Bestrophin-1 (Best1) and bestrophin-2 (Best2) are two members of the bestrophin family of calcium (Ca2+)-activated chloride (Cl−) channels with critical involvement in ocular physiology and direct pathological relevance. The bestrophins are a family of Ca2+-activated anion channels consisting of four members (Best1–4) in mammals. The overall architecture of hBest1 and hBest2 resembles the pentameric assembly previously shown by KpBest, cBest1 and bBest2, and retains the two landmark permeation constrictions, the neck and aperture, in the ion conducting pathway. Ample electrophysiological evidence indicates that the neck and aperture serve as dual Ca2+-dependent channel “gates”, as disrupting either of them partially impairs Ca2+-dependence while disrupting both makes the channel completely Ca2+-independent.

To elucidate the architecture of human bestrophins, we purified WT hBest1 and hBest2 for single-particle cryo-EM analysis in the absence of Ca2+ (EGTA), or after a 30 s spike of 1 μM or 5 mM Ca2+. Under both 1 μM and 5 mM Ca2+ conditions, most of the hBest1/hBest2 particles (~90–95%) were in a Ca2+-bound closed state, which is very similar to the Ca2+-unbound closed state. By comparing Ca2+-bound hBest2 in the closed and open states, we defined the structural changes coordinated with neck gating at residues 346–379. In the closed state, this region is well-ordered and wraps around the circumference of the cytosolic domain, extending clockwise around the channel when viewed from the membrane. Therefore, the binding of residues 346–379 to the channel periphery provides an inter-protomer cooperative mechanism to constrict the channel concentrically. The hBest2 aperture recapitulates structural features previously seen in bBest2: the K208-E212 pair, connected by a salt bridge, forms a constriction in the ion conduction pathway within the cytosolic region; an ion-like density is captured at the level of K208, possibly representing a passing Cl−. The high similarity between hBest2 and bBest2 structures suggests a critical involvement of K208-E212 in hBest2 channel gating and selectivity, as we previously reported for bBest2 K208-E21212. Interestingly, S205 of hBest2 adopts two conformations in the Ca2+-bound state, such that it can point directly into or away from the central axis, imposing a constriction with radius of 1.8 Å and 2.6 Å, respectively. As S205 is conserved in most mammalian Best2 homologs and Best2 is reported to conduct HCO3− 21, the dual conformation of S205 may affect the flow of larger anions.

>MTVTYTARVANARFGGFSQLLLLWRGSIYKLLWRELLCFLGFYMALSAAYRFVLTEGQKRYFEKLVIYCDQYASLIPVSFVLGFYVTLVVNRWWSQYLCMPLPDALMCVVAGTVHGRDDRGRLYRRTLMRYAGLSAVLILRSVSTAVFKRFPTIDHVVEAGFMTREERKKFENLNSSYNKYWVPCVWFSNLAAQARREGRIRDNSALKLLLEELNVFRGKCGMLFHYDWISVPLVYTQVVTIALYSYFLACLIGRQFLDPAQGYKDHDLDLCVPIFTLLQFFFYAGWLKVAEQLINPFGEDDDDFETNFLIDRNFQVSMLAVDEMYDDLAVLEKDLYWDAAEARAPYTAATVFQLRQPSFQGSTFDITLAKEDMQFQRLDGLDGPMGEAPGDFLQRLLPAGAGMVA[5x]> LAPSPQSPETPAPQNQTSRVVQAPKEEEEDEQEASEEKASEEEKAWLMASRQQLAKETSNFGFSLLRKISMRHDGNMVFSPFGMSLAMTGLMLGATGPTETQIKRGLHLQALKPTKPGLLPSLFKGLRETLSRNLELGLTQGSFAFIHKDFDVKETFFNLSKRYFDTECVPMNFRNASQAKRLMNHYINKETRGKIPKLFDEINPETKLILVDYILFKGKWLTPFDPVFTEVDTFHLDKYKTIKVPMMYGAGKFASTFDKNFRCHVLKLPYQG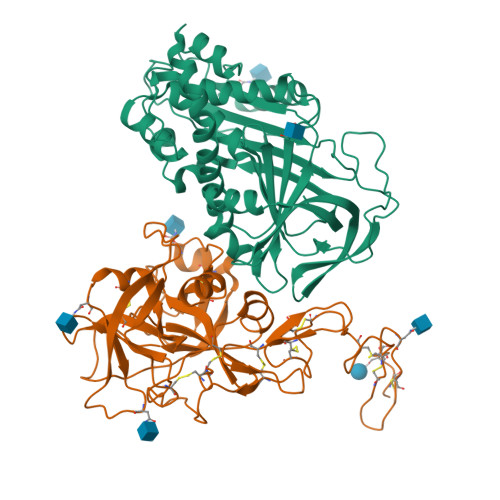NATMLVVLMEKMGDHLALEDYLTTDLVETWLRNMKTRNMEVFFPKFKLDQKYEMHELLRQMGIRRIFSPFADLSELSATGRNLQVSRVLQRTVIEVDERGTEAVAGILSEITAYSMPPVIKVDRPFHFMIYEETSGMLLFLGRVVNPTLL;> RYKGGSPCISQPCLHNGSCQDSIWGYTCTCSPGYEGSNCELAKNECHPERTDGCQHFCLPGQESYTCSCAQGYRLGEDHKQCVPHDQCACGVLTSEKRAPDLQDLPWQVKLTNSEGKDFCGGVIIRENFVLTTAKCSLLHRNITVKTYFNRTSQDPLMIKITHVHVHMRYDADAGENDLSLLELEWPIQCPGAGLPVCTPEKDFAEHLLIPRTRGLLSGWARNGTDLGNSLTTRPVTLVEGEECGQVLNVTVTTRTYCERSSVAAMHWMDGSVVTREHRGSWFLTGVLGSQPVGGQAHMVLVTKVSRYSLWFKQIMN(R)-4-AMINO-ISOXAZOLIDIN-3-ONE | C3 H6 N2 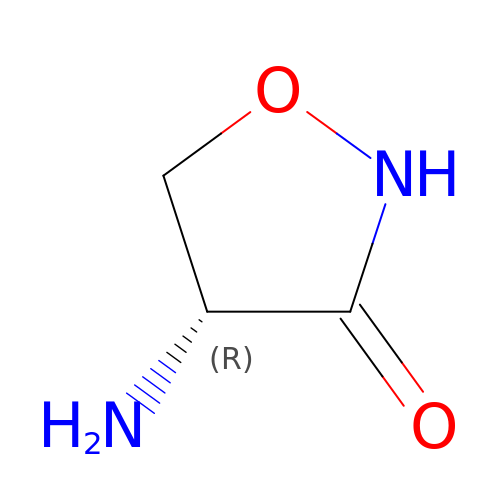O2 | DYDCUQKUCUHJBH-UWTATZPHSA-N>[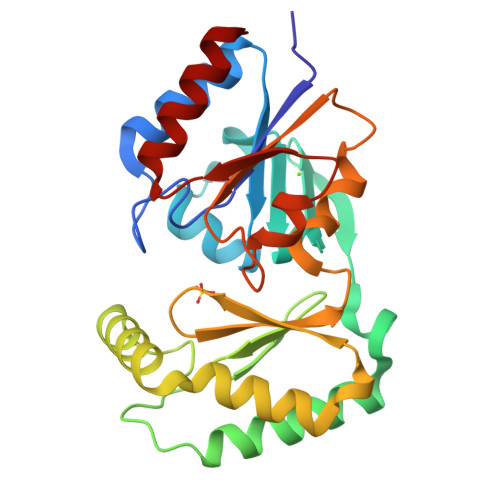2x]GMKRVLLLFDVDGTLTPPRLCQTDEMRALIKRARGAGFCVGTVGGSDFAKQVEQLGRDVLTQFDYVFAENGLLAYRNGLEIHRQSLLNALGNDRIVKFVKKTLRLIADLDIPVQRGTFVEYRNGMINVSPIGRNCSQAERDEFEVYDNEHRVRASLIAELENSFPDFGLKYSIGGQISFDVFPVGWDKTYCLQFVEDDFEEIHFFGDKTQEGGNDYEIYTDKRTIGHKVTSYKDTIAEVEKIIAMK>GSAPVTVTRFVDASPTGYDWRADWVKGFPIDSSCNATQYNQLSTGLQEAQLLAEHARDHTLRFGSKSPFFRKYFGNETASAEVVGHFDNVVGADKSSILFLCDDLDDKCKNDGWAGYWRGSNHSDQTIICDLSFVTRRYLTQLCSSGYTVSKSKTNIFWAGDLLHRFWHLKSIGQLVIEHYADTYEEVLELAQENSTYAVRNSNSLIYYALDVYAYDVTIPGEGCNGDGTSYKKSDFSSFEDSDSGSDSGASSTASSSHQHTDSNPSATTDANSHCHTHADGEVHC[6x]

In response to such conditions of low zinc availability, C. albicans secretes a zinc-scavenging protein called Pra1 to capture zinc from the host. Following extracellular secretion, Pra1 associates with the fungal cell via a cognate receptor called Zrt101; the PRA1 and ZRT101 genes are encoded at the same genetic locus. In this study, we present cryo-EM structures of C. albicans Pra1 in the apo-state as well as in the zinc-bound state at 2.8 Å and 2.5 Å resolution, respectively. The structure reveals a hexameric ring-like assembly in which each subunit is related to its neighbor by a 180° rotation.

From our cryo-EM structure of Pra1 prepared in the presence of 1 mM ZnSO4, we observe that the cryo-EM map is continuous amongst a cluster of three histidine residues (His 178, His 182 and His 193), which all point towards each other, consistent with the coordination of a metal ion. In this subunit (subunit B), the center of the zinc ion is equidistant to the center of the N3-nitrogen in the imidazole ring of each histidine residue. There is an extension of cryo-EM density in the metal ion binding site, likely indicating the presence of a water molecule to complete the tetrahedral coordination of the zinc ion. Although we generated two final maps for the Pra1:Zn2+ structure, one with c1 (no symmetry) and the other with three-fold c3 symmetry imposed, we analyzed and deposited the c1 map. In the c1 map, we are able to observe that the distances from the center of the zinc ion to the center of the N3-nitrogen in the histidine residue vary by subunit. For instance, in subunit A, the distance from the center of the zinc ion to the center of the N3-nitrogen of His 193 and His 182 is 2.3 Å. In contrast, the distance from the center of the zinc ion to the center of the N3-nitrogen of His 178 is 2.7 Å. These variations may be indicative of differential binding modes and may be important in the molecular mechanism of zinc ion binding by the Pra1 hexamer. In the context of the overall Pra1 architecture, these six Zn2+ binding sites are located on the outer face of the hexameric ring. The lack of metal ion coordination, and the change in pH, does not lead to global conformational changes in the resolved portions of Pra1. Indeed, a structural superposition of the hexamers in the presence and absence of Zn2+, shown in Supplementary Fig. 7, has an RMSD = 0.175 Å.> MSLGIRYLALLPLFVITACQQPVNYNPPATQVAQVQPAIVNNSWIEISRSALDFNVKKVQSLLGKQSSLCAVLKGDAYGHDLSLVAPIMIENNVKCIGVTNNQELKEVRDLGFKGRLMRVRNATEQEMAQATNYNVEELIGDLDMAKRLDAIAKQQNKVIPIHLALNSGGMSRNGLEVDNKSGLEKAKQISQLANLKVVGIMSHYPEEDANKVREDLARFKQQSQQVLEVMGLERNNVTLHMANTFATITVPESWLDMVRVGGIFYGDTIASTDYKRVMTFKSNIASINYYPKGNTVGYDRTYTLKRDSVLANIPVGYADGYRRVFSNAGHALIAGQRVPVLGKTSMNTVIVDITSL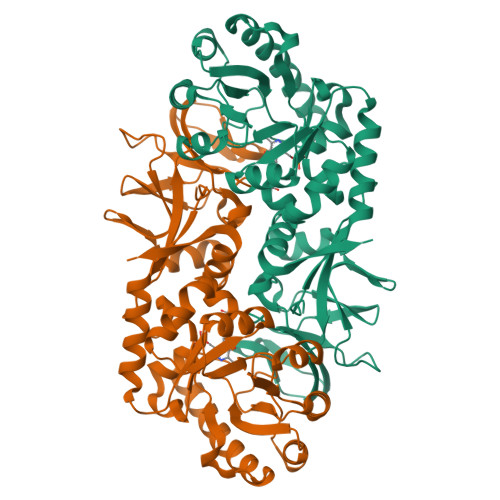NNIKPGDEVVFFGKQGNSEITAEEIEDISGALFTEMSILWGATNQRVLVD> 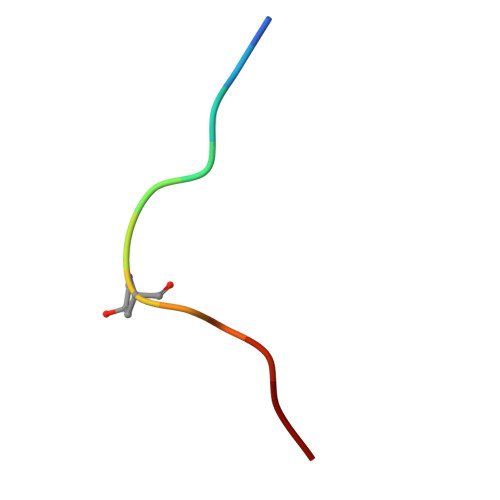HEVPSGPNPISN>KRKIIYLASPYGFSQQQKTLLLPPIVRALEALGIEVWEPFARNNQIDFSQADWAYRVAQADLQDVKNCDGIFAVVNGTPPDEGVMVELGMAIALNKAIFLFRDDFRRCSDNERYPLNLMLFAGLPEIGWENYYYTSVDEIQSHDKALYKWLTGM[2x]

Here, we characterize the structure and function of a thermophilic dNDT, the protein from Chroococcidiopsis thermalis (CtNDT). Nucleoside 2′-deoxyribosyltransferase (dNDT) enzymes catalyze transglycosylation via a covalent 2′-deoxyribosylated enzyme intermediate with retention of configuration, having applications in the biocatalytic synthesis of 2′-deoxynucleoside analogues in a single step. The reaction catalyzed by dNDT proceeds via a ping-pong mechanism, with the formation of a 2′-deoxyribosyl-enzyme intermediate covalently linked to an active-site glutamate.13 Transglycosylation occurs in a stereospecific manner, preserving the anomeric carbon in the β configuration in the newly formed 2′-deoxyribonucleoside. As with other NDT enzymes, the active site of CtNDT is formed by residues from two monomers, and therefore, it is only fully formed in the dimer/tetramer.

The structure of wild-type CtNDT was solved by molecular replacement with PHASER. The overall structure of CtNDT is similar to that of T. brucei nucleoside 2′deoxyribosyltransferase (TbNDT),61 as structural superposition reveals an RMSD of 0.859 Å. Size exclusion data reveal CtNDT to be a tetramer in solution formed by a dimer of dimers, which is also corroborated by the analysis of protein interfaces with PISA. Wild-type CtNDT was used as a search model for complex structures.>GAASMGPGRQVGDRSYYIGLLRPKITELTTEIERLNEQEELIVKGGSVLTQLQQRNKALTDEAAKLKGTLADINLALEKSTTQDPSSVKDQATKLNQVNGEKRKQVDQLFLNAKEMEALTKKNTQALEEEMQNLDRRILAENQDFGLYKATRDEAFNVSDAVLSHQHQIRMLTAKQELLMTKLSTDPDKKRAAEVLRGILSKRQLKEELTKQCALSVEEERQLLIKQVKTARGDIEVLERQVNETRDALSESKNRCASLDEELKSYSGDNIKAFQELQEKDRELQSFMDSFPAKLKEEMDKITEVQRNIATLLERISQALELKKQMPQ[2x];>GAASMRQNPPKEPSEEEVLQYIVDNVNKLLSRHYSLVEFDAIQGTDLLQILADIFGTLSPAQQIDMGVAPTDEAAASMLEFLTKTLGYRVPPMLADSFPTSFSRAEPTVIYPTLYWVLSNMQQNEKRVYLARFLQRLEIPEAMLAQDEDVRALYQQYVNLRGMFVNTHRRVDALRTAHADPADARRAVTVLEEECDRLRGYIQVAEKKLAGVPDKEALLNACKSLRAALEEESRLAEKGVELQQQLISSRQRSTEMHNRLQNLRRDAADGRVDVIVRRLRDEIQTNKMIIEEQLPKELQQKQRENAEFDRLISEPLDMQALTTENQQLDEALKKLHQQVKERQKPGEDGSTIATIKQQVERVAKR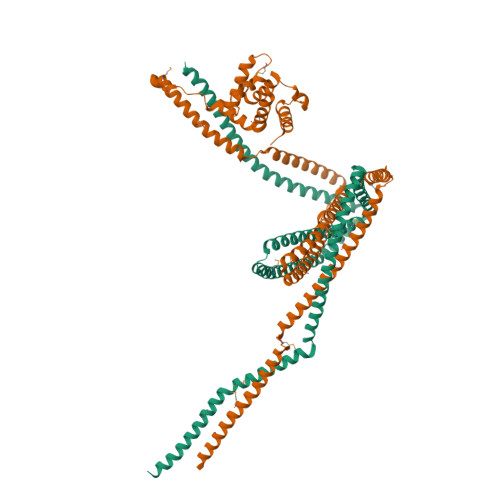KVEVMEQLTGLQADNSRTLNDIRERENRIEQLREAHHMLKDDDFREFSKQVLAKKAATESMRTHLSEQRVEYGVLNFTENVLRSQFTSL[2x];> MSDDLVKILVLGPSKSGKSTVTNFLAGTRDTPTKEYHETNPLRVLEVEIALDDTRRSGRQAAGLKKAVVQLWDVGGSSKHQAGWPAIASNADGIIYVFNPEVKGSEKELLLWYKNFALNQDELDDDNNFKMRVTDGHSLIFSHHSSLPEFAVGDNAIPPMPPKQLQGIRALETSLDYQSDNFKEAFDALVEQIIASRLAAEENDLLQKEREAKDYPRLKR> MGLTGLEIYKHLPKKNCKECGQPTCLAFAMQIAAGKAGLDACPYVSDEAKELLESASAPPVALIKVGKGEKVLEIGHETVLFRHDKRFEHPCGLAILVEDTLSEGEIKERVEKINKLVFDRVGQMHSVNLVALKGSSQDAATFAKAVATAREVTDLPFILIGTPEQLAAALETEGANNPLLYAATADNYEQMVELAKKYNVPLTVSAKGLDALAELVQKITALGYKNLILDPQPENISEGLFYQTQIRRLAIKKLFRPFGYPTIAFALDENPYQAVMEASVYIAKYAGIIVLNTVEPADILPLITLRLNIYTDPQKPIAVEPKVYEILNPGPDAPVFITTNFSLTYFCVAGDVEGARIPAYILPVDTDGTSVLTAWAAGKFTPEKIAQFLKESGIAEKVNHRKAILPGGVAVLSGKLQELSGWEILVGPRESSGINSFIKQ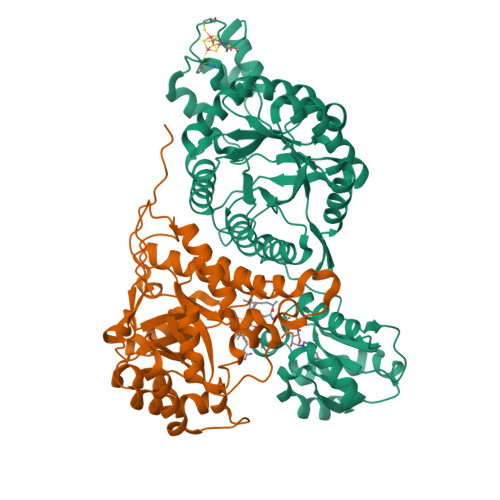RWNV;> MAVEVLKEKWNSKVVEVTLGTGDKTVTLGGDSTLPFLTFEGEMPNPPRFALEVFDTPPTDWPDILVEPFKDVINDPVAWAKKCVEYGADIVALRLVSAHPDGQNRSGAELAEVCKAVADAIDVPLMIIGCGVEEKDAEIFPVIGEALSGRNCLLSSATKDNYKPIVATCMVHGHSVVASAPLDINLSKQLNIMIMEMNLAPNRIIMDPLIGALGYGIEYSYSIIERMRLGALTGDKILAMPVVCFIGQEAWKAKEAKDPEVAEWGDYALRAIHWETVTTVALIQAGGHLFVMRHPKSLAEVKEHLKRILK>FTEGTDYMVLEKPIPNADKTLIKVFSYACPFCYKYDKAVTGPVSEKVKDIVAFTPFHLETKGEYGKQASEVFAVLINKDKAAGISLFDANSQFKKAKFAYYAAYHDKKERWSDGKDPAAFIKTGLDAAGMSQADFEAALKEPAVQETLEKWKASYDVAKIQGVPA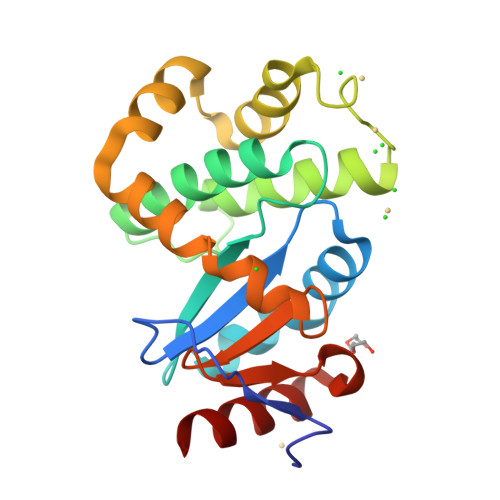YVVNGKYLIYTKSIKSIDAMADLIRELASK[2x]> AAPSFDCGKPQVEPKKCPGRVVGGCVAHPHSWPWQVSLRTRFGMHFCGGTLISPEWVLTAAHCLEKSPRPSSYKVILGAHQEVNLEPHVQEIEVSRLFLEPTRKDIALLKLSSPAVITDKVIPACLPSPNYVVADRTECFITGWGETQGTFGAGLLKEAQLPVIENKVCN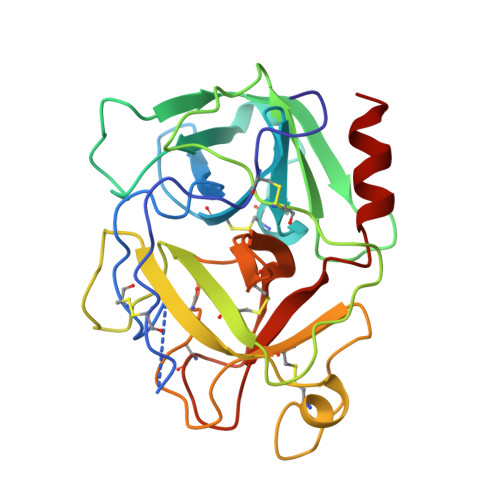RYEFLNGRVQSTELCAGHLAGGTDSCQGDAGGPLVCFEKDKYILQGVTSWGLGCARPNKPGVYVRVSRFVTWIEGVMRNN>[3x]GGRDKDHLLKYNVG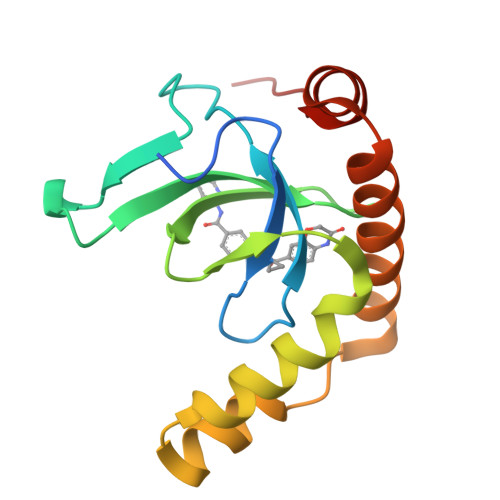DLVWSKVSGYPWWPCMVSADPLLHSYTKLKGQKKSARQYHVQFFGDAPERAWIFEKSLVAFEGEGQFEKLCQESAKQAPTKAEKIKLLKPISGKLRAQWEMGIVQAEEAASMSVEERKAKFTFLYVG(1~{S},10~{S})-12-cyclopropyl-1-oxidanyl-10-propan-2-yl-9,12-diazatricyclo[8.2.1.0^{2,7}]trideca-2(7),3,5-trien-11-one | C17 H22 N2 O2 | 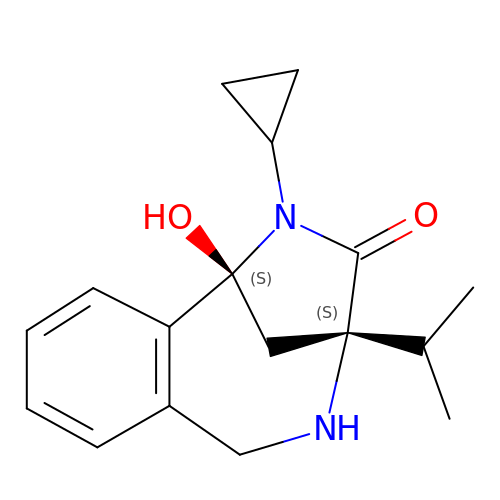JXXKUMYBOLYKNF-IRXDYDNUSA-N5-methyl-7-oxo-6-(propan-2-yl)-4,7-dihydropyrazolo[1,5-a]pyrimidine-3-carbonitrile 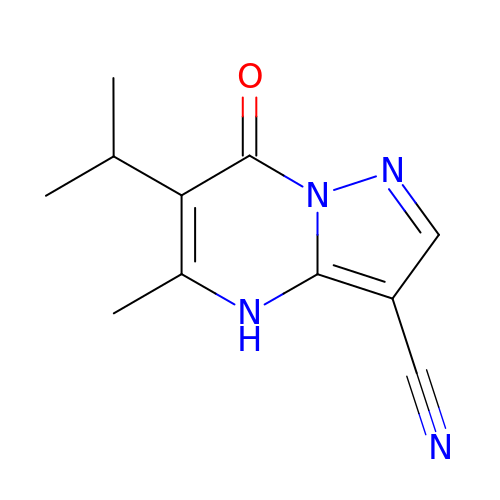| C11 H12 N4 O | UHVUUCAAVHIPKM-UHFFFAOYSA-N>[264x]MYTNSDFVVIKALEDGVNVIGL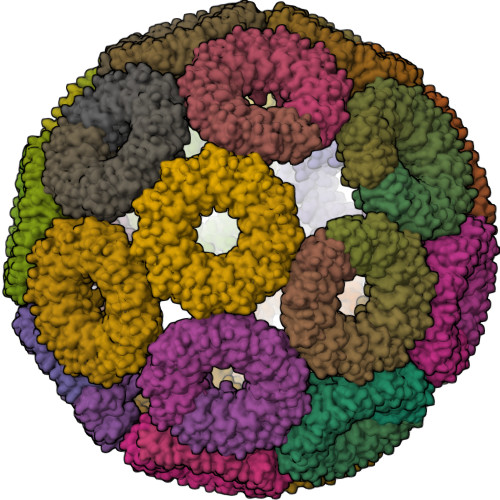TRGADTRFHHSECLDKGEVLIAQFTEHTSAIKVRGKAYIQTSHGVIESEGKK> GSVKIGHYILGDTLGVGTFGKVKVGKHELTGHKVAVKILNRQKIRSLD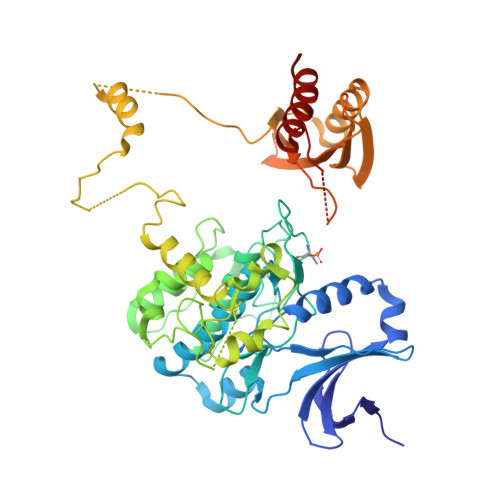VVGKIRREIQNLKLFRHPHIIKLYQVISTPSDIFMVMEYVSGGELFDYICKNGRLDEKESRRLFQQILSGVDYCHRHMVVHRDLKPENVLLDAHMNAKIADFGLSNMMSDGEFLRTSCGSPNYAAPEVISGRLYAGPEVDIWSSGVILYALLCGTLPFDDDHVPTLFKKICDGIFYTPQYLNPSVISLLKHMLQVDPMKRASIKDIREHEWFKQDLPKYLFPEDPSYSSTMIDDEALKEVCEKFECSEEEVLSCLYNRNHQDPLAVAYHLIIDNRRIMNEAKDFYLATSPPDSFLDDHHLTRPHPERVPFLVAETPRARHTLDELNPQKSKHQGVRKAKWHLGIRSQSRPNDIMAEVCRAIKQLDYEWKVVNPYYLRVRRKNPVTSTYSKMSLQLYQVDSRTYLLDFRSIDDGITAAASGTATPQRSGSVSNYRSCQRSDSDAEAQGKSSEVSLTSSVTSLDSSPVDLTPRPGSHTIEFFEMCANLIKILAQ>[2x]MEKFLVIAGPCAIESE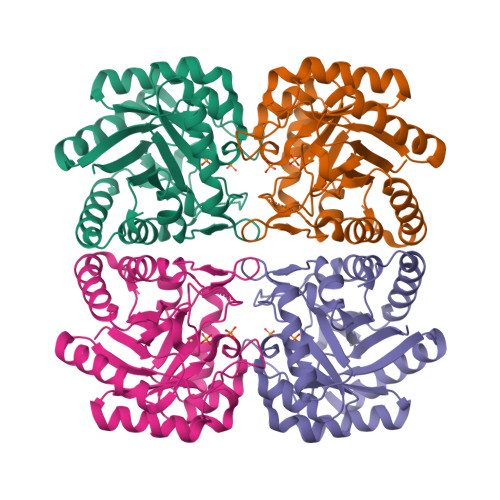ELLLKVGEEIKRLSEKFKEVEFVFKSSFDKANRSSIHSFRGHGLEYGVKALRKVKEEFGLKITTDIHESWQAEPVAEVADIIQIPAFLCRQTDLLLAAAKTGRAVNVKKGQFLAPWDTKNVVEKLKFGGAKEIYLTERGTTFGYNNLVVDFRSLPIMKQWAKVIYDATGSVQLPGGLGDKSGGMREFIFPLIRAAVAVGCDGVFMETHPEPEKALSDASTQLPLSQLEGIIEAILEIREVASKYYETIPVK>[4x]GGFNRFEAAKLVMQWLCNHEDQNMQRMAVAIISILAAKLSTEQTAQLGTELFIVRQLLQIVKQKTNQNSVDTTLKFTLSALWNLTDESPTTCRHFIENQGLELFMRVLESFPTESSIQQKVLGLLNNIA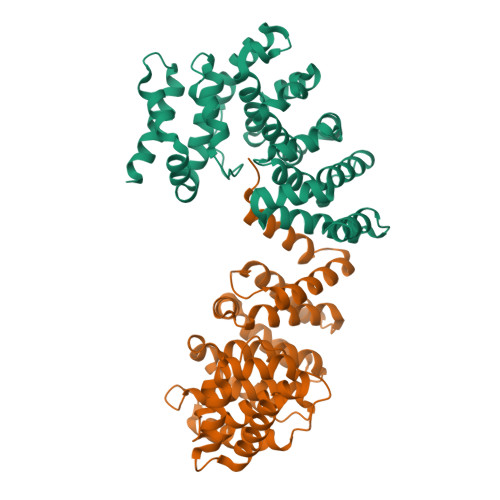EVQELHSELMWKDFIDHISSLLHSVEVEVSYFAAGIIAHLISRGEQAWTLSRSQRNSLLDDLHSAILKWPTPECEMVAYRSFNPFFPLLGCFTTPGVQLWAVWAMQHVCSKNPSRYCSMLIEEGGLQHLYNIKDHEHTDPHVQQIAVAILDSLEKHIVR>MGSSHHHHHSSGENLYFQGHMKKQLIEFVRWSPERAQHYRNKGYWIDQPLTRILTVGVQSHPHSLAIICGERQLSYIELDRLSTNLATRLAEKGLGKGDTALVQLPNVAEFYIVFFALLKAGVVVLNALYSHRQYELNAFIKQIQPKLLIGSRQHEVFSNNQFIDSLHDVNLSPEIILMLNHQATDFGLLDWIETPAETFVDFSSTPADEVAFFQLSGGSTGTPKLIPRTHNDYDYSVRASAEICGLNSNTRLLCALPAPHNFMLSCPGALGVLHAGGCVVMAPNPEPLNCFSIIQRHQVNMASLVPSAVIMWLEKAAQYKDQIQSLKLLQVGGASFPESLARQVPEVLNCKLQQAFGMAEGLVNYTRLDDSDEQIFTTQGRPISSDDEIKIVDEQYREVPEGEIGMLATRGPYTFCGYYQSPEHNSQVFDEDNYYYSGDLVQRTPDGNLRVVGRIKDQINRGGEKIASEEIEKLILLHPEVMHAALVAIVDEQFGEKSCAFIVSRNPELKAVVLRRHLMELGIAQYKLPDQIKLIESLPLTAVGKVDKKQLRSILNTSTTS[2x]

Acinetobacter baumannii produces the catecholate siderophore acinetobactin to scavenge iron, a nutrient essential for several metabolic processes. The biosynthesis begins with BasE, a standalone adenylation domain, which activates and loads 2,3-dihydroxybenzoic acid (DHB) to the phosphopantetheinyl arm of the PCP domain of BasF. Adenylation domains have two subdomains, a large N-terminal subdomain (Acore) and a smaller C-terminal subdomain (Asub), which is highly dynamic, adopting unique conformations to carry out each individual step of the adenylation reaction. Several binding pocket residues were identified within 5 Å of the ligand, including Asn242, Phe243, Ser247, Val336, Val344, and Tyr346.

We solved the structures of the V336A and V336G mutants, which showed a general improvement in activity with the C4-substituted substrates from our panel and the structure of the V336A/S247C double mutant, which showed some of the highest activities among our mutants bound to 4-fluorosalicylic acid. Finally, the most dramatic improvements in catalytic efficiency were observed for the double mutant V336A/S247C, which had a ∼40-fold improvement for 4-fluorosalicylic acid and a ∼100 fold improvement for 4-methylsalicylic acid. The activities of this double mutant with 4-fluorosalicylic acid and 4-methylsalicylic acid were comparable to that of WT BasE with its native substrate DHB. These improvements in catalytic efficiencies were mainly attributed to the significant reduction in apparent KM observed with the mutants indicating that the mutagenesis likely improved the binding affinities of these substrates. The mutant S247C and the double mutant S247C/V336A showed reduced catalytic efficiency for DHB by more than 10-fold. The double mutant had significantly higher activity for salicylic acid (∼3-fold) emphasizing the importance of the hydrogen bond formation between the Ser247 and the C3 position hydroxyl group of DHB. We then analyzed the structure of the double mutant V336A/S247C, which exhibited both an increase in space in the binding pocket and the introduction of the cysteine residue observed in aryl adenylating enzymes that bind salicylate. This mutant demonstrated some of the highest increases in specific activity and showed improved catalytic efficiencies with the 4-substituted analogs, comparable to WT BasE for DHB. When combined with mutations that switch the specificity code of BasE to prefer salicylic acid, this activity can be further improved and be comparable to the activity of the WT enzyme with its native substrate DHB.>MTSLEIAIIVAIVLVIAIAVGWYLYTTFAAAGQQTGLTATKATIYVTKDGNVYLNVTLVPQGAAQVAISSIEVAGVSIPCTSSNLVKAPGEYVIELSSVSVSVGQVLTGRIVLASGAISPFTATVVAADHVPSTENKLCSSQ[41x]

We present in this paper the structure of two additional archaeal T4P, one from Pyrobaculum arsenaticum, a neutrophilic hyperthermophile (optimal growth at 90 °C, pH 7) and the other from Saccharolobus solfataricus, an acidophilic hyperthermophile (optimal growth at 75–80 °C, pH 2-3). Although the full spectrum of functions played by archaeal T4P is yet to be uncovered, they are known to mediate adhesion to various biotic and abiotic surfaces, and play an important role in DNA exchange, intercellular communication and biofilm formation. Finally, we show that Pyrobaculum and the Saccharolobus T4P are at the forefront of virus-host interaction and are recognized by two different viruses, likely serving as primary receptors during virus infection. We show that whereas the N-terminal domain is conserved in all bacterial and archaeal T4P-like filaments, the C-terminal domain of bacterial T4P is unrelated to the immunoglobulin (Ig)-like domain shared by archaeal T4P and archaeal flagella.

In contrast, the sequence identity between the pilins from P. arsenaticum and S. solfataricus is only ~18%. In contrast, ~10% of the residues in P. arsenaticum pilin are charged. Interestingly, and in contrast to the S. islandicus and S. solfataricus pilins, P. arsenaticum pilin has a 15 amino acid C-terminal extension that wraps around the globular domain. Within this extension, an intramolecular disulfide bond is formed between Cys139 in the extension and Cys80 within the same pilin chain, which is likely to contribute to the thermo-stability of this pilus. In S. solfataricus, we see clear extra density consistent with glycosylation on seven residues, all serines or threonines. In contrast, in P. arsenaticum only a single density consistent with glycosylation is seen, on Asn55, which would be N-linked glycosylation. First, although T4P of a neutrophilic P. arsenaticum is as hydrophobic as those of acidophilic S. islandicus and S. solfataricus, it does not possess the extensive sugar coating. Instead, T4P of P. arsenaticum is stabilized by an intramolecular disulfide bond, a protein adaptation to high temperatures previously reported in bacteria, archaea and their viruses. Consistent with this prediction, boiling the S. islandicus pili in 5 M GuHCl failed to disassemble the filaments, but under the same conditions the P. arsenaticum pili come apart. Interestingly, Iho670 adhesion filament packs very similarly to S. solfataricus and S. islandicus pili, with an RMSD < 2 Å, while P. arsenaticum packs slightly differently from those three filaments with RMSDs of 3–4 Å. Notably, the crucial N-terminal subunit-subunit interactions in these four filaments are almost all hydrophobic, except for in P. arsenaticum there is a glutamic acid, which may contribute to the slightly different packing compared to Iho670 and other archaeal T4P.> PSQMEHAMETMMFTFHKFAGDKGYLTKEDLRVLMEKEFPGFLENQKDPLAVDKIMKDLDQCRDGKVGFQSFFSLIAGLTIAC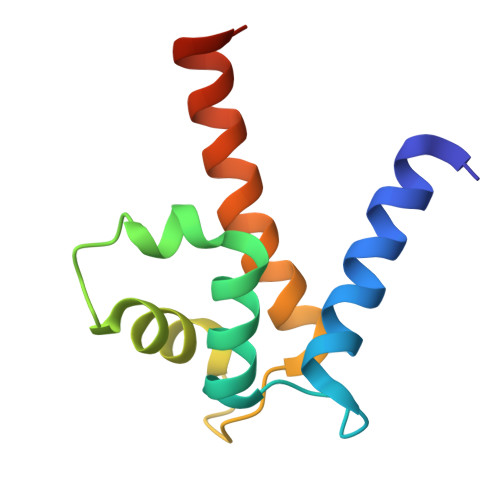NDYFVVHMKQKGKK>SIQVIARAASIMRALGSHPHGLSLAAIAQLVGLPRSTVQRIINALEEEFLVEALGPAGGFRLGPALGQLINQAQTDILSLVKPYLRSLAEELDESVSLASLAGDKIYVLDRIVSERELRVVFPIGINVPAAATAAGKVL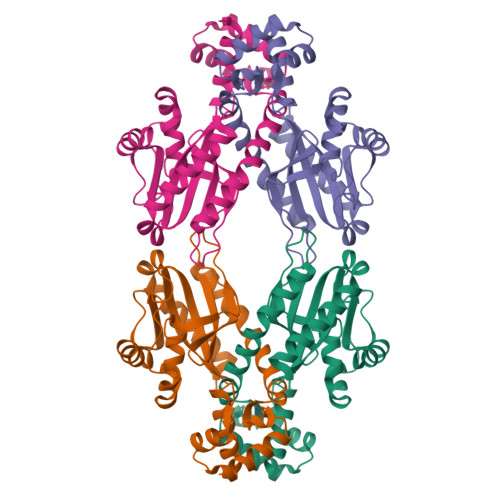LAALPDETLQAALGEQLPVLTSNTLGRKALVKQLSEVRQSGVASDLDEHIDGVSSFATLLDTYLGYYSLAIVMPSSRASKQSDLIKKALLQSKLNIERAIGR[2x]>[4x]MAHHHHHHVGTDDWRCARSMHEFSLKDIDGHMVNLDKYRGFVCILTNVASQCG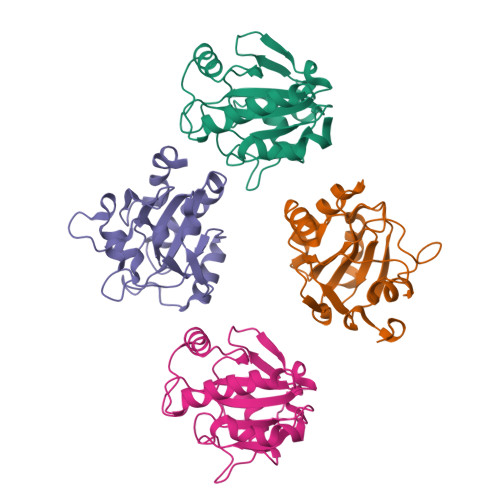KTEVNYTQLVDLHARYAECGLRILALPCNQFGKQEPGSNEEIKEFAAGYNVKFDMFSKVCVNGDDAHPLLKWMKIQPKGKGILGNAIKWNFTKFLIDKNGCVVKRYGPMEEPLVIEKDLPHYF11-methyl-3-(pyridin-3-ylmethyl)-4H-pyrimido[5'',4'':5',6']pyrido[2',3':4,5]pyrimido[1,2-b]pyridine-4,6(3H)-dione | C20 H14 N6 O2 | 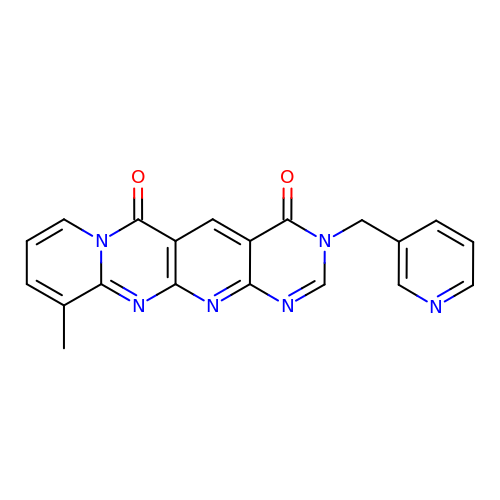BFJYZGRLIJMXES-UHFFFAOYSA-N The Cafeteria roenbergensis virus (Crov), Dictyostelium, and other species encode a large family of leucine-rich repeat (LRR) proteins with FGxxFN motifs. The FGxxFN repeat proteins belong to a larger family termed FNIP proteins (Pfam PF05725), which in turn appear related to the large and well-studied Leucine-rich repeat (LRR) family of proteins. The structures reveal a so far unique hydrophobic packing with a buried phenylalanine spine and thus define a new sub-class of LRR proteins. We now report the first structures, namely those of Crov588 and Crov537. Their perhaps most striking structural feature is a fully buried double phenylalanine spine that originates from their diagnostic FGxxFN motifs.

Crov539 and Crov527 represent the second sub-class of the here analyzed repeat proteins with an LxxLxFGxxFNQPIExVxW/LPxx consensus (supplementary sequence file). We crystallized Crov539 and solved its structure by molecular replacement using a homology model based upon the Crov588 structure. Crov539 has a short and curved core comprising 12 regularly shaped repeats. This core is flanked by a compact 15-residue N-terminal capping module. At the C-terminus, a unique domain swapping arrangement occurs where the last repeat(s) (261–290) of the first molecule extends across and caps another molecule to form a dimer. Dimerization is also evident in gelfiltration experiments. For both the Crov527 and Crov539 repeats, the packing within the hydrophobic core is altered through a substitution of the LP motif for WP at positions 19–20. The restriction between prolines 13 and 20 and the inclusion of a bulky tryptophan residue gives rise to a reversal of the hydrophobic core packing at residues 17 and 18. Unlike Crov588, Crov539 lacks the histidine ladder derived from position 3 of the repeat as this residue is almost exclusively threonine. Residue 5 on the concave surface of the repeat is uncharged and either threonine at the N-terminus of the structure or isoleucine (Ile110, Ile134, Ile156, Ile180, Ile202) towards the C-terminal region, creating a hydrophobic patch at the center of the lower concave surface.

>[6x]GSMTLVIKTNEDLNKLNDNIHTLTIGANFNQPIEHIKWPKLLTTLTFEWYFDQPIENVKLPDSLTTLTFGYSFNQPIEKVKWPKTLAFLTFGYKFNKPIEKVKWPDSLTTLIFEENSLFDQSIEKIKWSNSLTTLIFGWNFNQPIENVEWPESLTTLVFNEDSIFNQPIENVKWPKLLKTIIFGCHFNHPIENVKWPGSLTTLIFGDDFNQPFENVILPKSLTNLTFGPNFNQPLNFLPESLKNITITTNYQQNLYNLPSSLNCIKIISYKRTYEHIVNVLPEHLKKKVIKI> LYFQGAMALEEIKNGTDISTLDIRKFNLNINNVSVLSKSQSVDQFHLSNPHYEYLSGGAYPGEMENFTLKVDKSKKQDQVFENPLSLKFTNIGTVNGKQVDAYLNFNKVTLHYLNTAQAESEMNSAQKSTVEFFSISELWESNAFEIGNVPYVDANHDYIMNKAFWIDADVTAEIRYADGTETDLKLVMKPTDIDAIDANNLKETFYVKNYQNDVNLRLMNNANVLVQEEASDRTSWIATQITGGSYNENNVSGLALRSNSNSMNFGYSSTETCSAVFGLYIEKIDPR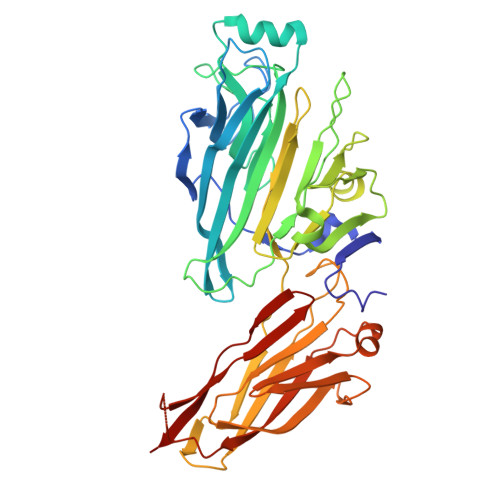PVLEVDPAEIPAKDGQDVTYKATFKVPVPGKDILAAPSSIEMVQKFDERLDYKELKVESGGVTLQEGRDYTIEKTGQTVTVKMTPEYLKGNSSSDIIITYKTATNKKVEEKGSEKIDNTVTLHVDNLSAPSNQVSTALLYEK> MDETGKELVLALYDYQEKSPREVTMKKGDILTLLNSTNKDWWKVEVGDRQGFVPAAY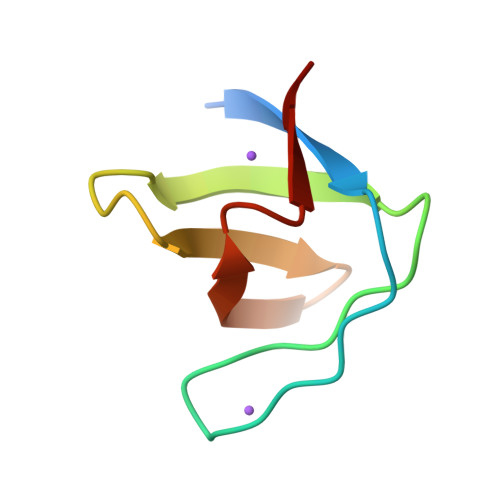VKKLD> MDYKDDDDKSQKNGIATLLQAE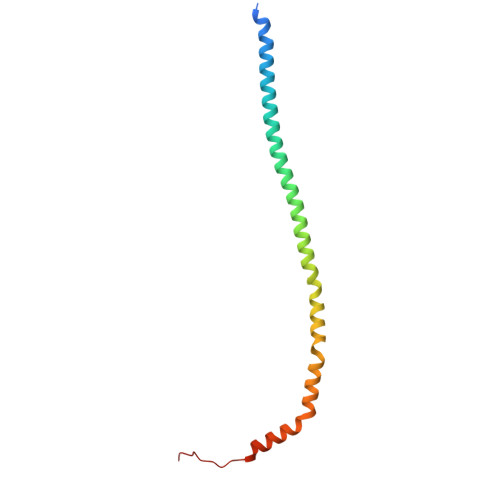KEAHEIVSKARKYRQDKLKQAKTDAAKEIDSYKIQKDKELKEFEQKNAGGVGELEKKAEAGVQGELAEIKKIAEKKKDDVVKILIETVIKPSAEVHINAL> MSAYATQGFNLDDRGRRIVVDPVTRIEGHMRCEVNVDANNVIRNAVSTGTMWRGLEVILKGRDPRDAWAFVERICGVCTGCHALASVRAVENALDIRIPKNAHLIREIMAKTLQVHDHAVHFYHLHALDWVDVMSALKADPKRTSELQQLVSPAHPLSSAGYFRDIQNRLKRFVESGQLGPFMNGYWGSKAYVLPPEANLMAVTHYLEALDLQKEWVKIHTIFGGKNPHPNYLVGGVPCAINLDGIGAASAPVNMERLSFVKAR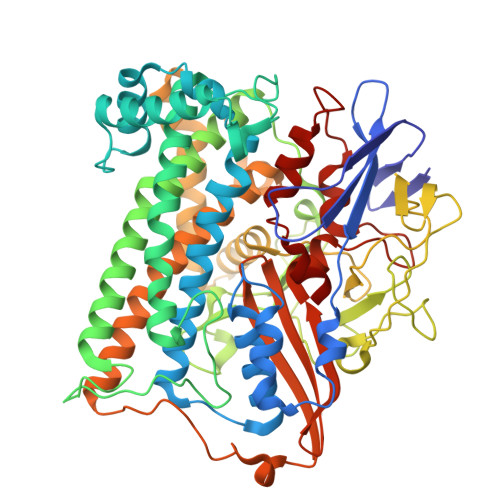IDEIIEFNKNVYVPDVLAIGTLYKQAGWLYGGGLAATNVLDYGEYPNVAYNKSTDQLPGGAILNGNWDEVFPVDPRDSQQVQEFVSHSWYKYADESVGLHPWDGVTEPNYVLGANTKGTRTRIEQIDESAKYSWIKSPRWRGHAMEVGPLSRYILAYAHARSGNKYAERPKEQLEYSAQMINSAIPKALGLPETQYTLKQLLPSTIGRTLARALESQYCGEMMHSDWHDLVANIRAGDTATANVDKWDPATWPLQAKGVGTVAAPRGALGHWIRIKDGRIENYQCVVPTTWNGSPRDYKGQIGAFEASLMNTPMVNPEQPVEILRTLHSFDPCLACSTH>[6x]PKPGDIFEVELAKNDNSLGISVTGGVNTSVRHGGIYVKAVIPQGA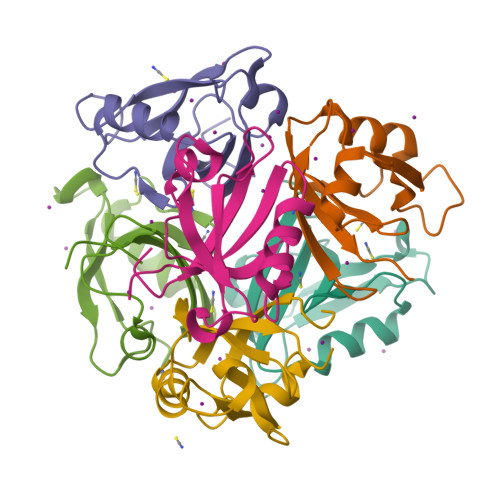AESDGRIHKGDRVLAVNGVSLEGATHKQAVETLRNTGQVVHLLLEKGQSPT>PPYIFSPIPFLGHAIAFGKSPIEFLENAYEKYGPVFSFTMVGKTFTYLLGSDAAALLFNSKNEDLNAEDVYSRLTTPVFGKGVAYDVPNPVFLEQKKMLKSGLNIAHFKQHVSIIEKETKEYFESWGESGEKNVFEALSELIILTASHCLHGKEIRSQLNEKVAQLYADLDGGFSHAAWLLPGWLPLPSFRRRDRAHREIKDIFYKAIQKRRQSQEKIDDILQTLLDATYKDGRPLTDDEVAGMLIGLLLAGQHTSSTTSAWMGFFLARDKTLQKKCYLEQKTVCGE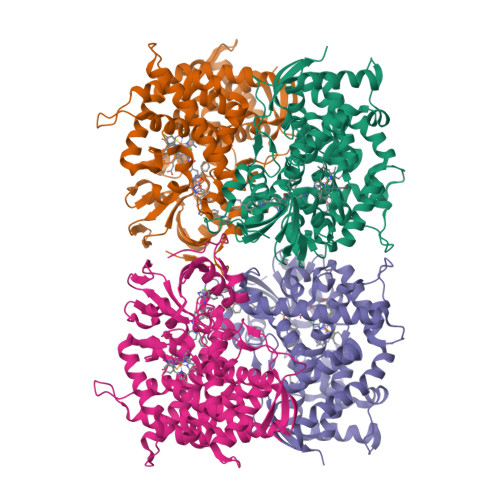NLPPLTYDQLKDLNLLDRCIKETLRLRPPIMIMMRMARTPQTVAGYTIPPGHQVCVSPTVNQRLKDSWVERLDFNPDRYLQDNPASGEKFAYVPFGAGRHRCIGENFAYVQIKTIWSTMLRLYEFDLIDGYFPTVNYTTMIHTPENPVIRYKRRSK[4x]>SNAMFKIKTIESLSDLTQLKKAYFDSSIVPLDGMWHFGFAPMAKHFGFYVNKNLVGFCCVNDDGYLLQYYLQPEFQLCSQELFTLISQQNSSVIGEVK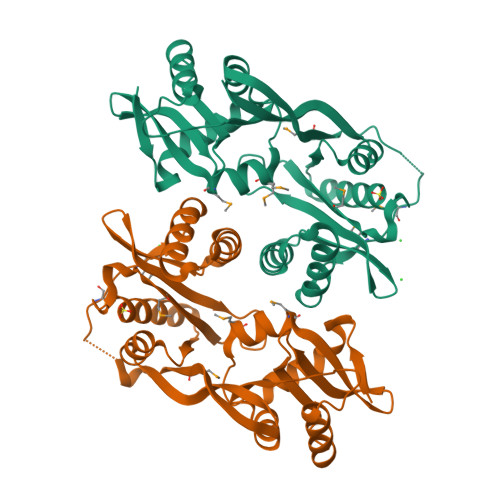GAFVSTAELNYQALCLDNSATFKVNSLMYQHNTKLADRNLEMIDMQIAGTEQLTAFVTFAAANIGAPEQWLTQYYGNLIERKELFGYWHKGKLLAAGECRLFDQYQTEYADLGMIVAQSNRGQGIAKKVLTFLTKHAATQGLTSICSTESNNVAAQKAIAHAGFTSAHRIVQFEFKHA[2x]>[35x]HEFAELFYRTYIVTPDQAGFQLSIRRNLVWEGWTGEGLSGEKQEISKRNILQGLLDYTTLETNSTELIPVIQSGENDEQFIDPSVLPAQTVKQGKDTFDTNFLKFSENGEGFNLLMLAQTPSRLKKGSMTFTDSLDSRIALKQLLISVTKGGTTELFALDVNRDQYAAYTATREYNFRLMQLKFHTSLGLGEESTTVAGAESALLKDLFDLGYRIELDVKVDGEMNVENGNGDTSLRALRLARVFDKEGKEIALTDSRVSAALSGLTVTGVGYSLEARLTNINQLEMGLLIDSDVQKQGFMIPTLPPLVIVKPAMVEDDKTYPRLEALTTAYRIQQMRNNAVTTLLNRADTLKSYLGVGVPHPIESNLGLEGVGQYYVRPYYNEATIDVLNDLNNLTSAAKQTDIQGLIVSKINEMVYTADQLTGYTAALEAAFSGRSPKPHVAIGTDM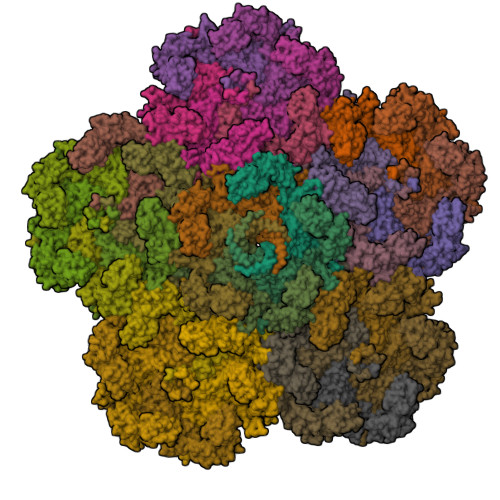RLPQYIQINGDDRTVGIGYDYTIARISDLRMKDKIVMTFILPNESEPHPLQHGVLGFIPEYLVDFNMIRNQRIGREIRLTPRYRYFNFLPIMLVINVINLEEAIAQRTALDVNETQVTPAS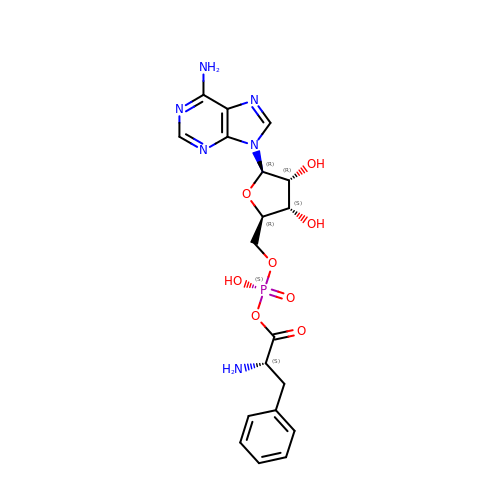ADENOSINE-5'-[PHENYLALANINYL-PHOSPHATE] | C19 H23 N6 O8 P | ZFNOOEXYTZPIQS-URQYDQELSA-N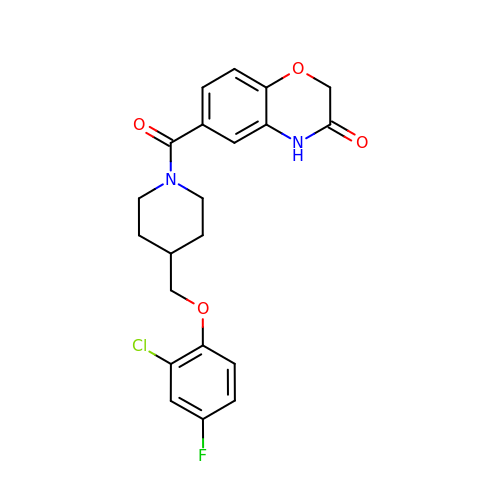6-{4-[(2-chloro-4-fluorophenoxy)methyl]piperidine-1-carbonyl}-2H-1,4-benzoxazin-3(4H)-one | C21 H20 Cl F N2 O4 | UUUUFICXTVCJQV-UHFFFAOYSA-N> GKPGLDDPLPTERLASEHLKPGCQGEQCPLVNIDTLKFPDEPQLDPIVERALLEMTRE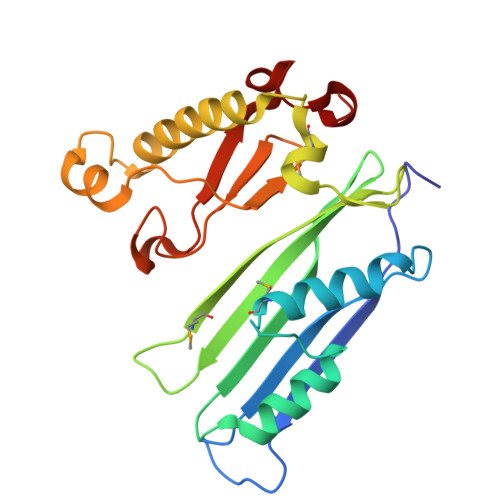NNETPLPASLAAYERQFLDSAEPGWSSYLQAKVREQHDGLVIIELSSYLFTGGAHGMPGRGFINYDRRQHKVLSLQDMLVPGQEEAFWKQAELAHKAWLLANKLDQDADFQKTWPFQRTPHVALTFGAVTLKYDAYSIAPYSYAHPELKIPYPRLNGIVKPNLFPGRG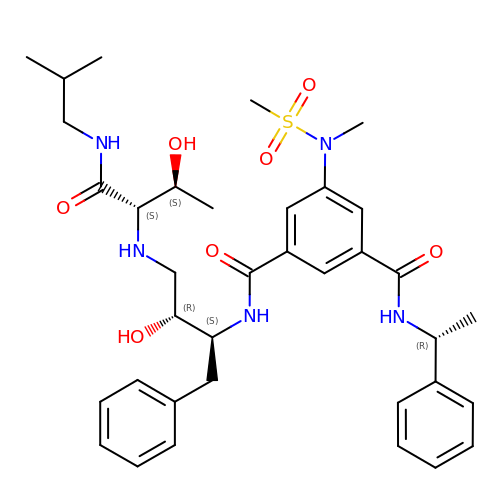N-[(2S,3R)-3-hydroxy-4-({(2S,3S)-3-hydroxy-1-[(2-methylpropyl)amino]-1-oxobutan-2-yl}amino)-1-phenylbutan-2-yl]-5-[methyl(methylsulfonyl)amino]-N'-[(1R)-1-phenylethyl]benzene-1,3-dicarboxamide | C36 H49 N5 O7 S | ZIEVAMMZKBNDFB-AAZBAGLXSA-N>PMFIVNTNVPRASVPDGFLSELTQQLAQATGKPPQYIAVHVVPDQLMAFGGSSEPCALCSLHAIGKIGGAQNRSYSKLLCGLLA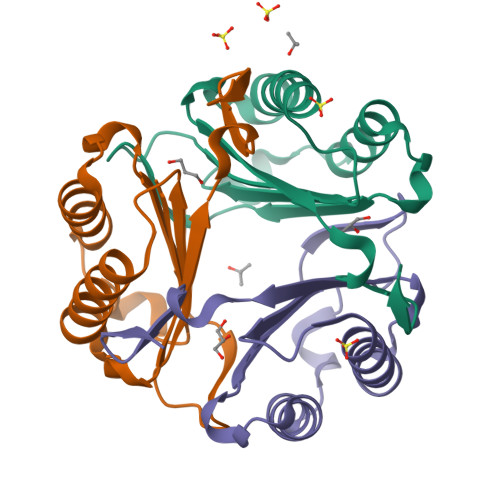ERLRISPDRVYINYYDMNAANVGWNNSTFA[3x]> GEFTQSVSRLQSIVAGLKNAPSDQLINIFESCVRNPVENIMKILKGIGETFCQHYTQSTDEQPGSHIDFAVNRLKLAEILYYKILETVMVQETRRLHGMDMSVLLEQDIFHRSLMACCLEIVLFAYSSPRTFPWIIEVLNLQPFYFYKVIEVVIRSEEGLSRDMVKHLNSIEEQILESLAWSHDSALWEALQVSANKVPTCEEVIFPNNFETGRPKRTGSLALFYRKVYHLASVRLRDLCLKLDVSNELRRKIWTCFEFTLVHCPDLMKDRHLDQLLLCAFYIMAKVTKE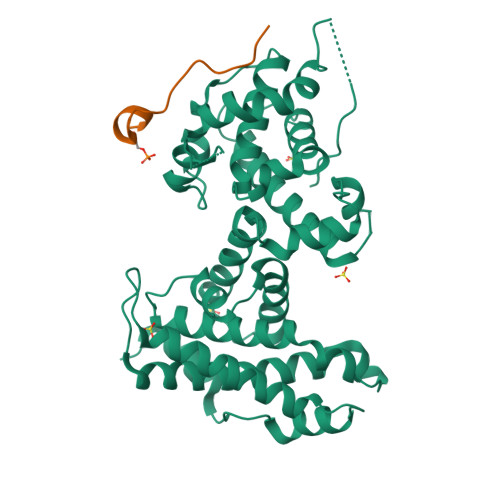ERTFQEIMKSYRNQPQANSHVYRSVLLKSIKEERGDLIKFYNTIYVGRVKSFALKYDLANQDHMMDAPPLSPFPHIKQQ;> EASLLSFEKLDRASADLWPE>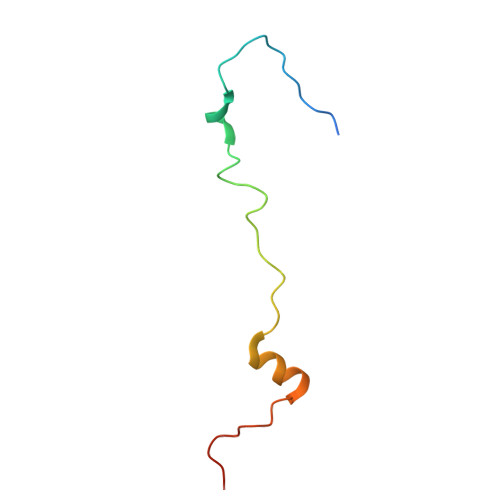 MANFDGNEMRGMTHANYEDSRLNKSRELNANMSIGTSKSEDEYGRQVHSLTKQSYSDDSVQEA> MSYLLTSALLFALGVYGVLTRRTAILVFLSIELMLNAAN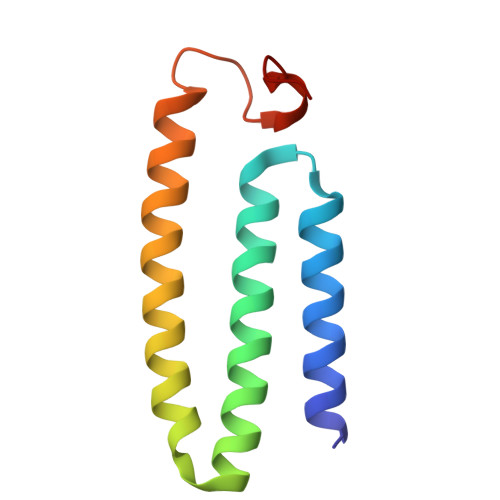LSLVGFARAYGLDGQVAALMVIAVAAAEVAVGLGLIVAIFRHRESTAVDDLSELRG>[4x]LWPWPQNFQTSDQRYVLYPNNFQFQYDVSSAAQPGCSVLDEAFQRYRDLLFGSGSWPRPYLTGKRHTLEKNVLVVSVVTPGCNQLPTLESVENYTLTINDDQCLLLSETVWGALRGLETFSQLVWKSAEGTFFINKTEIEDFPRFPHRGLLLDTSRHYLPLSSILDTLDVMAYNKLNVFHWHLVDDPSFPYESFTFPELMRKGSYNPVTHIYTAQDVKEVIEYARLRGIRVLAEFDTPGHTLSWGPGIPGLLTPCYSGSEPSGTFGPVNPSLNNTYEFMSTFFLEVSSVFPDFYLHLGGDEVDFTCWKSNPEIQDFMRKKGFGEDFKQLESFYIQTLLDIVSSYGKGYVVWQEVFDNKVKIQPDTIIQVWREDIPVNYMKELELVTKAGFRALLSAPWYLNRISYGPDWKDFYVVEPLAFEGTPEQKALVIGGEACMWGEYVDNTNLVPRLWPRAGAVAERLWSNKLTSDLTFAYERLSHFRCELLRRGVQAQPLNVGFCEQEFEQT;>[4x]AKPGPALWPLPLSVKMTPNLLHLAPENFYISHSPNSTAGPSCTLLEEAFRRYHGYIFGFYKWHHEPAEFQAKTQVQQLLVSITLQSECDAFPNISSDESYTLLVKEPVAVLKANRVWGALRGLETFSQLVYQDSYGTFTINESTIIDSPRFSHRGILIDTSRHYLP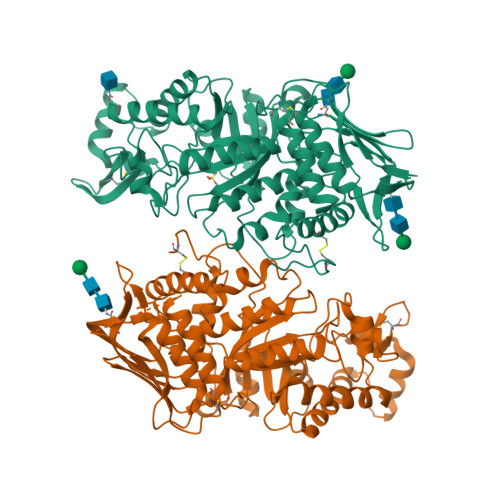VKIILKTLDAMAFNKFNVLHWHIVDDQSFPYQSITFPELSNKGSYSLSHVYTPNDVRMVIEYARLRGIRVLPEFDTPGHTLSWGKGQKDLLTPCYSRQNKLDSFGPINPTLNTTYSFLTTFFKEISEVFPDQFIHLGGDEVEFKCWESNPKIQDFMRQKGFGTDFKKLESFYIQKVLDIIATINKGSIVWQEVFDDKAKLAPGTIVEVWKDSAYPEELSRVTASGFPVILSAPWYLDLISYGQDWRKYYKVEPLDFGGTQKQKQLFIGGEACLWGEYVDATNLTPRLWPRASAVGERLWSSKDVRDMDDAYDRLTRHRCRMVERGIAAQPLYAGYCNHENM(1~{R},3~{R})-5-[(2~{E})-2-[(4~{a}~{R},5~{S},9~{a}~{S})-4~{a}-methyl-5-[(2~{R})-6-methyl-6-oxidanyl-heptan-2-yl]-3,4,5,6,7,8,9,9~{a}-octahydro-2~{H}-benzo[7]annulen-1-ylidene]ethylidene]-2-(3-oxidanylpropylidene)cyclohexane-1,3-diol | C31 H52 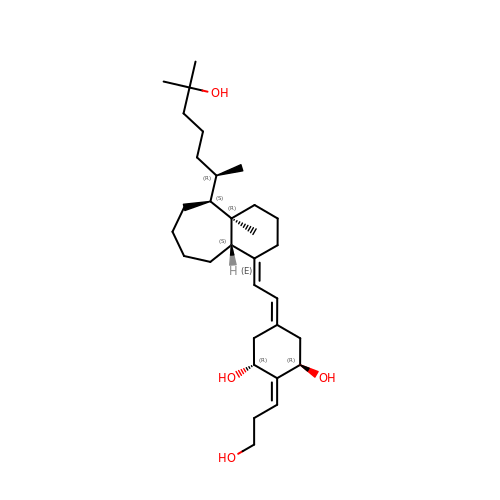O4 | UMSSGYONEBAMGL-DNSSBSRKSA-N>[2x]C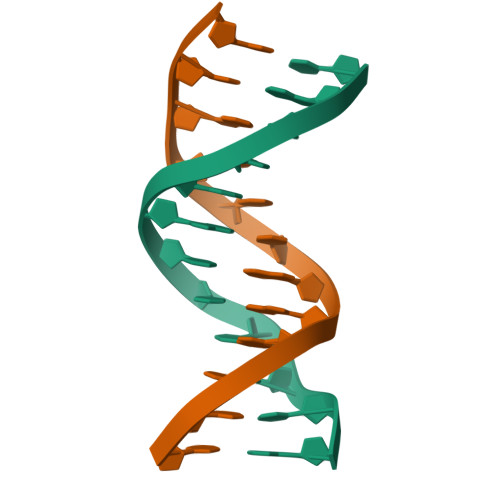GCGAATTCXCG> SQTIALLNIYRNPQNSSQSADGLRSAVSDVEMQEHYDEFFEEVFTEMEEKY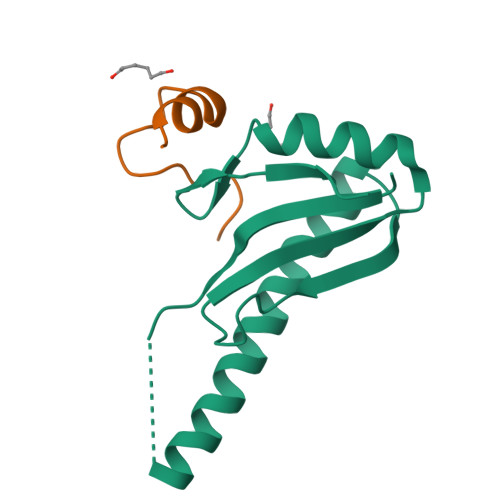GEVEEMNVCDNLGDHLVGNVYVKFRREEDAEKAVIDLNNRWFNGQPIHAELSP;> KKKVRKYWDVPPPGFEHITPMQYKAMQA> ITGYAACPRNWIGVGNKCFYFSEYASNWTFSQ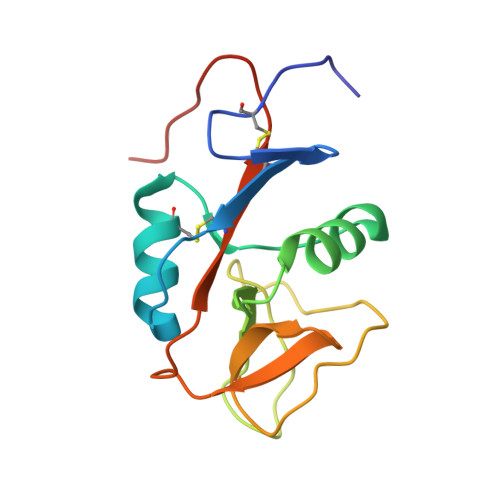TFCKAQEAELARFDTEEELNFLSRYKGSFDYWIGLHRESSEHPWKWTDNTQYNYSLSIRGVERYAYLNDIGISSARVYADKRWSCSRLNSGTHHHHHHHHG> MNNMNVIIADDHPIVLFGIRKSLEQIEWVNVVGEFEDSTALINNLPKLDAHVLITDLSMPGDKYGDGITLIKYIKRHFPSLSIIVLTMNNNPAILSAVLDLDIEGIVLKQGAPTDLPKALAALQKGKKFTPESVSRLLEKISAGGYGDKRLSPKESEVLRLFAEGFLVTEIAKKLNRSIKTISSQKKSAMMKLGVENDIAL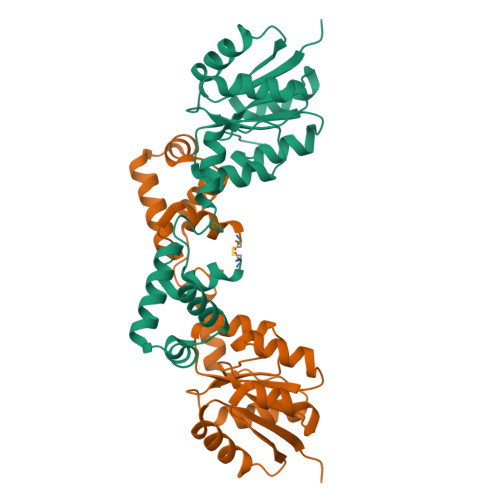LNYLSCVTL>MDTSLAEEVQQTMATLAPNRFFFMSPYRSFTTSGCFARFDEPAVNGDS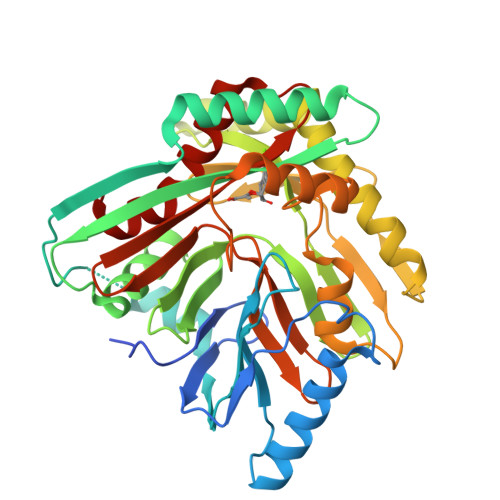PDSPFQQKLAALFADAKAQGIKNPVMVGAIPFDPRQPSSLYIPESWQSFSRQEKQASARRFTRSQSLNVVERQAIPEQTTFEQMVARAAALTATPQVDKVVLSRLIDITTDAAIDSGVLLERLIAQNPVSYNFHVPLADGGVLLGASPELLLRKDGERFSSIPLAGSARRQPDEVLDREAGNRLLASEKDRHEHELVTQAMKEVLRERSSELHVPSSPQLITTPTLWHLATPFEGKANSQENALTLACLLHPTPALSGFPHQAATQVIAELEPFDRELFGGIVGWCDSEGNGEWVVTIRCAKLRENQVRLFAGAGIVPASSPLGEWRETGVKLSTMLNVFGLH[2x]>[2x]AADEPQLLHGAGICKWFNVRMGFGFLSMTARAGVALDPPVDVFVHQSKLHMEGFRSLKEGEAVEFTFKKSAKGLESIRVTGPGGVFCIGSERRPKGGDRCYNCGGLDHHAK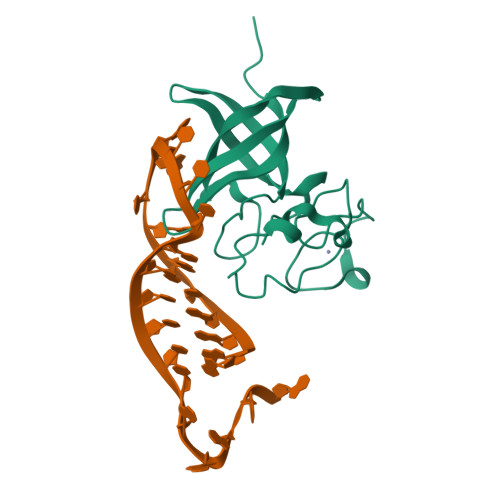ECKLPPQPKKCHFCQSISHMVASCPLKAQQGPSAQGK> MSESVTQQVFNFAVTKSQPFGGYVYSTNLTASTSSAVTSTQLTPLNLSITLGQITLSGNSLVIPATQIWYLTDAYVSVPDYTNITNGAEADGVILIYKDGVKLMLTTPLISSMSISNPARTHLAQAVKYSPQSILTMYFNPTK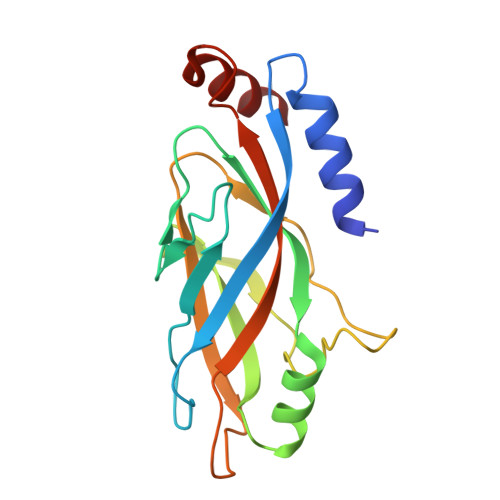PATASTSYPNTVYFTVVVVDFSYAQNPARAVVSANAVM>GAMGSGGGGEHQHGEEMMAAVPAPDAEGAAGFDEFPIGEDRDVGPLHVGGVYFQPV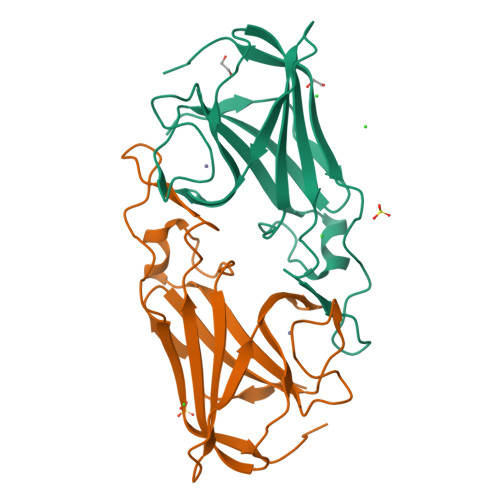EMHPAPGAQPSKEEADCHIEADIHANEAGKDLGYGVGDFVPYLRVVAFLQKHGSEKVQKVMFAPMNAGDGPHYGANVKFEEGLGTYKVRFEIAAPSHDEYSLHIDEQTGVSGRFWSEPLVAEWDDFEWKGPQW[2x]>GPTNNLLFKPPVESHIQKNKKILKSAKDLPPDALIIEYRGKFMLREQFEANGYFFKRPYPFVLFYSKFHGLEMCVDARTFGNEARFIRRSCTPNAEVRHEIQDGTIHLYIYSIHSIPKGTEITIAFDF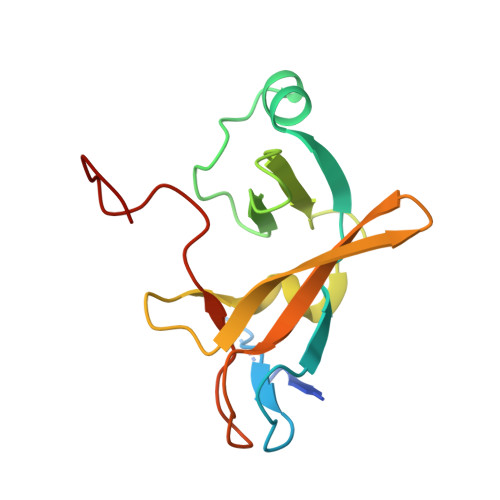DYGNAKYKVD[2x]> XRQCSM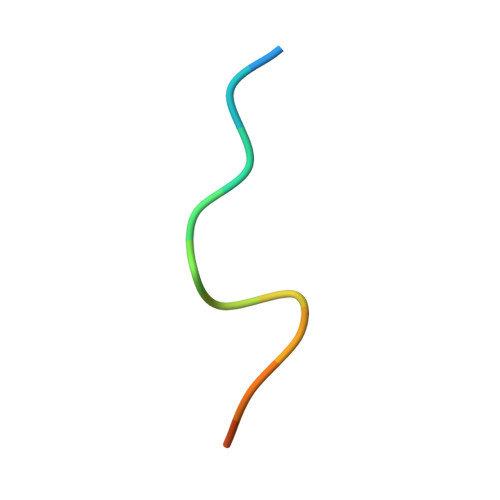TCFYHSKX> MG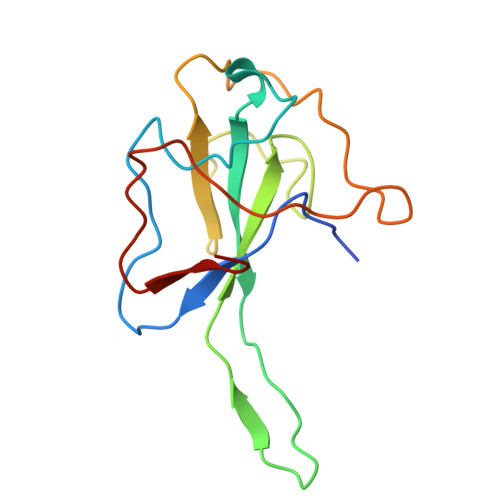SVVPHYSWFSGITQFQKGKEFQFAEGQGVPIANGIPASEQKGYWYRHNRRSFKTPDGQQKQLLPRWYFYYLGTGPHAGASYGDSIEGVFWVANSQADTNTRSDIVERDPSSHEAIPTRFAPGTVLPQGFYVEGSGRS(2S,5R,8R,11S,14S,17S,21R)-5,8,11,14,17-PENTAMETHYL-4,7,10,13,16,19-HEXAOXADOCOSANE-2,21-DIOL | C21 H44 O8 | 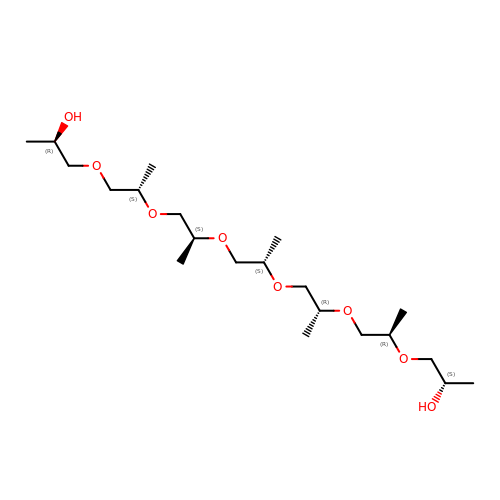XGDXHSHOQKNIEW-YSPFXGIPSA-N> MDAKARNCLLQHREALEKDIKTSYIMDHMISDGFLTIS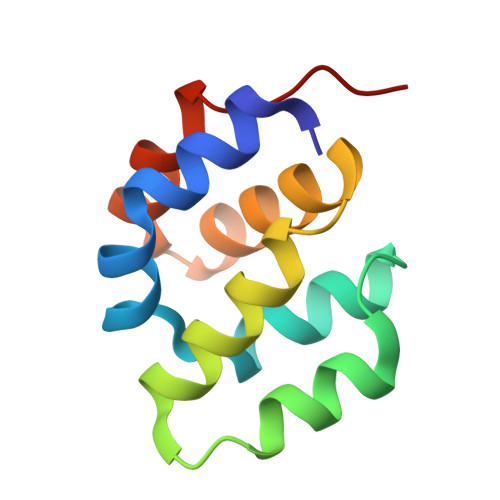EEEKVRNEPTQQQRAAMLIKMILKKDNDSYVSFYNALLHEGYKDLAALLHDGIPVVSSS> GHMSALFEPYTLKDVTLRNRIAIPPMCQYMAEDGMINDWHHVHLAGLARGGAGLLVVEATAVAPEGRITPGCAGIWSDAHAQAFVPVVQAIKAAGSVPGIQIAHAGRKASANRPWEGDDHIAADDTRGWETIAPSAIAFGAHLPKVPREMTLDDIARVKQDFVDAARRARDAGFEWIELHFAHGFLGQSFFSEHSNKRTDAYGGSFDNRSRFLLETLAAVREVWPENLPLTARFGVLEYDGRDEQTLEESIELARRFKAGGLDLLSVSVGFTIPDTNIPWGPAFMGPIAERVRREAKLPVTSAWGFGTPQLAEAALQANQLDLVSV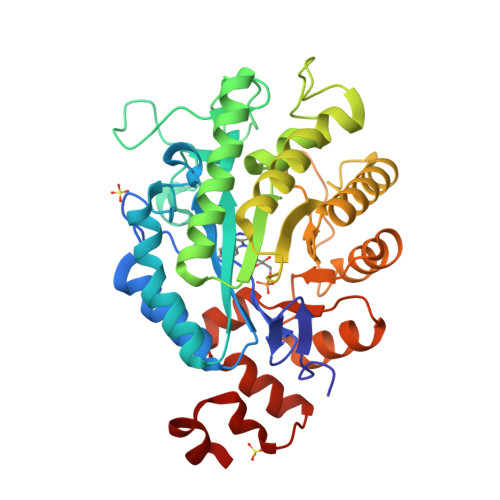GRAHLADPHWAYFAAKELGVEKASWTLPAPYAHWLERYR> GSQIPASEQETLVRPK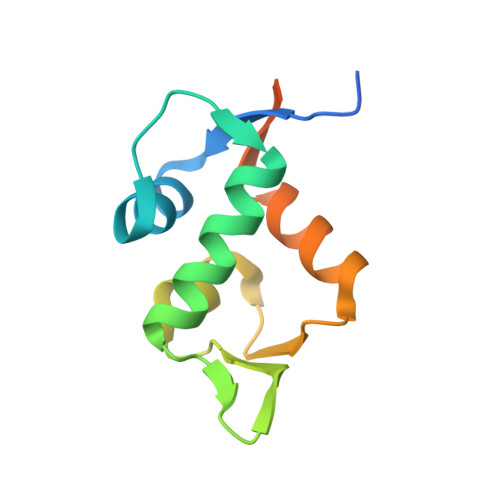PLLLKLLKSVGAQKDTYTMKEVLFYLGQYIMTKRLYDEKQQHIVYCSNDLLGDLFGVPSFSVKEHRKIYTMIYRNLVVVNQQESSDSGTSVSEN>ATTYNAVVSKSSSDGKTFKTIADAIASAPAGSTPFVILIKNGVYNERLTITRNNLHLKGESRNGAVIAAATAAGTLKSDGSKWGTAGSSTITISAKDFSAQSLTIRNDFDFPANQAKSDSDSSKIKDTQAVALYVTKSGDRAYFKDVSLVGYQATLYVSGGRSFFSDCRISGTVDFIFGDGTALFNNCDLVSRYRADVKSGNVSGYLTAPSTNINQKYGLVITNSRVIRESDSVPAKSYGLGRPWHPTTTFSDGRYADPNAIGQTVFLNTSMDNHIYGWDKMSGKDKNGNTIWFNPEDSRFFEYKSYGAGATVSKDRRQLTDAQAAEYTQSK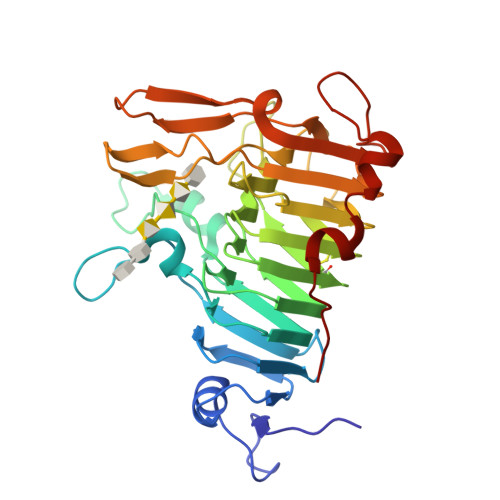VLGDWTPTLP[2x]>[6x]DELYRQSLEIISRYLREQATGAKDTKPMGRSGATSRKALETLRRVGDGVQRNHETA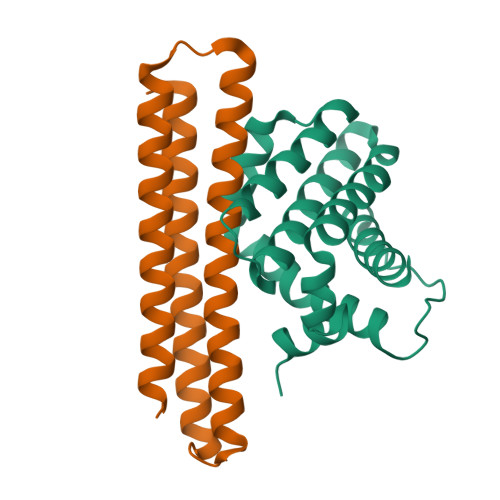FQGMLRKLDIKNEDDVKSLSRVMIHVFSDGVTNWGRIVTLISFGAFVAKHLKTINQESCIEPLAESITDVLVRTKRDWLVKQRGWDGFVEFFHVEDLEGGIRNVLLAFAGVAGVGAGLAYLIR;>[6x]DPKKVLDKAKDQAENRVRELKQVLEELYKEARKLDLTQEMRKKLIERYAAAIIRAIGDINNAIYQAKQEAEKLKKAGLVNSQQLDELLRRLDELQKEASRKANEYGREFELKLEYG(1R,2R,3R,4S,5R)-4-amino-5-[(R)-methylsulfinyl]cyclopentane-1,2,3-triol 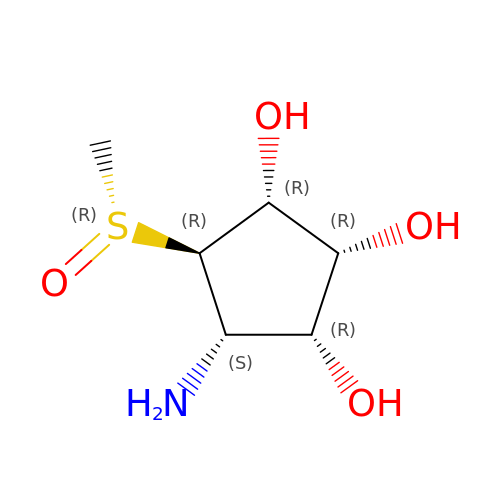| C6 H13 N O4 S | ZJFKRRRXLLAUHQ-DMRLTRFVSA-N>[2x]MEEPEEPADSGQSLVPVYIYSPEYVSMCDSLAKIPKRAS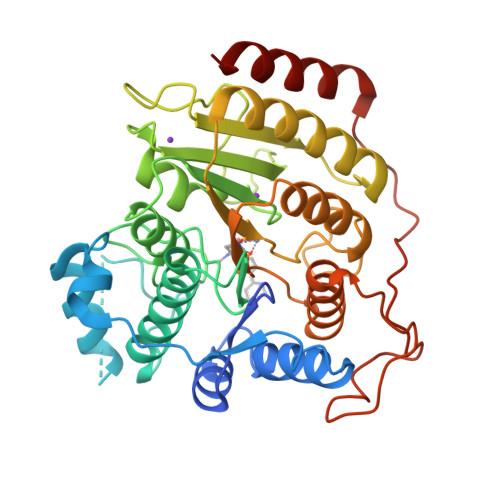MVHSLIEAYALHKQMRIVKPKVASMEEMATFHTDAYLQHLQKVSQEGDDDHPDSIEYGLGYDCPATEGIFDYAAAIGGATITAAQCLIDGMCKVAINWSGGWHHAKKDEASGFCYLNDAVLGILRLRRKFERILYVDLDLHHGDGVEDAFSFTSKVMTVSLHKFSPGFFPGTGDVSDVGLGKGRYYSVNVPIQDGIQDEKYYQICESVLKEVYQAFNPKAVVLQLGADTIAGDPMCSFNMTPVGIGKCLKYILQWQLATLILGGGGYNLANTARCWTYLTGVILGKTLSSEIPDHEFFTAYGPDYVLEITPSCRPDRNEPHRIQQILNYIKGNLKHVV> TLKY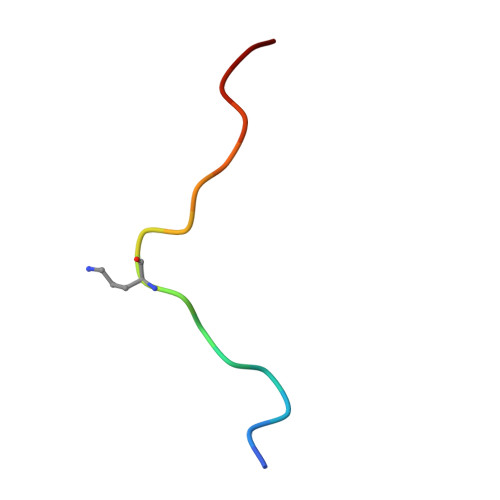PIEAGIVTNWDD> MNKNDHPLSHLFDNNDAWVKRKLADDPQYFSRLADQQAPEYLWIGCSDSRVPANQIIGLPPGEVFVHRNIANVVVHTDLNCLSVIQFAVDLLKVKHVMVVGHYGCSGVNAALHNRRVGLADNWLHHVQDVREKHAALLEDWPLGEARYRRLIELNAIEQVVNVCRTTIVNDAWARGQPL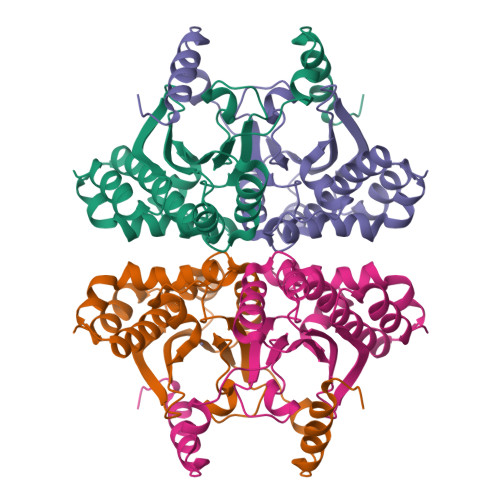TVHALVYGVHDGRMRNLGMAVSHAEQLDATYRRAVAALSASGAHSADNDVVAADAAQLAGAVDLIAQTIKETKHDGC> MNYTKFDVKNWVRREHFEFYRHRLPCGFSLTSKIDITTLKKSLDDSAYKFYPVMIYLIAQAVNQFDELRMAIKDDELIVWDSVDPCFTVFHQETETFSALSCPYSSDIDQFMVNYLSVMER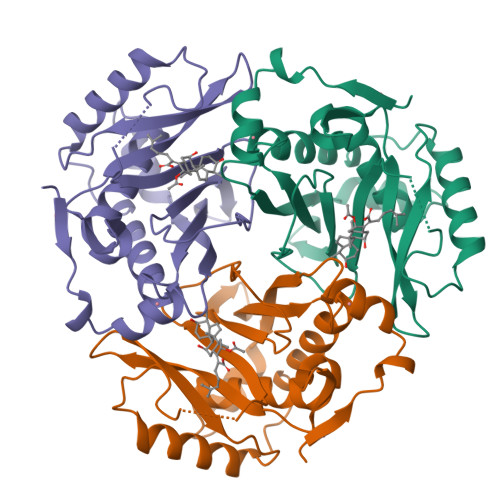YKSDTKLFPQGVTPENHLFISALPWVNFDSFNLNVANFTDFFAPVITMAKYQQEGDRLLLPLSVQVHHAVCDGFHVARFINRLQELCNSKLK>[2x]NDQLVELAKDPANWVMTGRDYNAQNYSEMTDINKENVKQLRPAWSFSTGVLHGHEGTPLVVGDRMFIHTPFPNTTFALDLNEPGKILWQNKPKQNPTARTVACCDVVNRGLAYWPGDDQVKPLIFRTQLDGHIVAMDAETGETRWIMENSDIKVG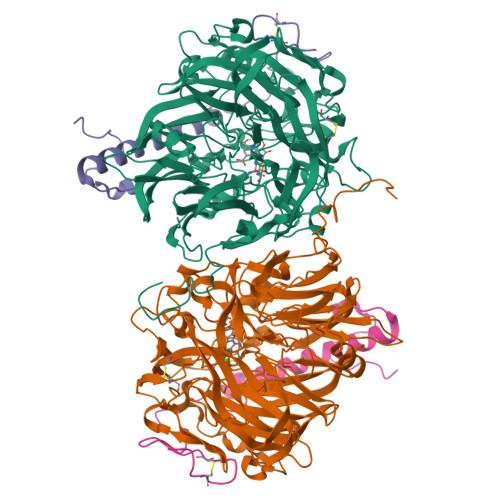STLTIAPYVIKDLVLVGSSGAELGVRGYVTAYDVKSGEMRWRAFATGPDEELLLAEDFNAPNPHYGQKNLGLETWEGDAWKIGGGTNWGWYAYDPEVDLFYYGSGNPAPWNETMRPGDNKWTMAIWGREATTGEAKFAYQKTPHDEWDYAGVNVMMLSEQEDKQGQMRKLLTHPDRNGIVYTLDRTNGDLISADKMDDTVNWVKEVQLDTGLPVRDPEFGTRMDHKARDICPSAMGYHNQGHDSYDPERKVFMLGINHICMDWEPFMLPYRAGQFFVGATLTMYPGPKGDRGNASGLGQIKAYDAISGEMKWEKMERFSVWGGTMATAGGLTFYATLDGFIKARDSDTGDLLWKFKLPSGVIGHPMTYKHDGRQYVAIMYGVGGWPGVGLVFDLADPTAGLGSVGAFKRLQEFTQMGGGVMVFSLDGESPYSDPNVGEYAPGEPT;>[2x]YDGTNCKAPGNCWEPKPDYPAKVEGSKYDPQHDPAELSKQGESLAVMDARNEWRVWNMKKTGKFEYDVKKIDGYDETKAPPAE>MAHHHHHHIPVTHIKCLRINGQIKCVKPISPNTTPAAEHIEHVRKNPRRKAAMDRA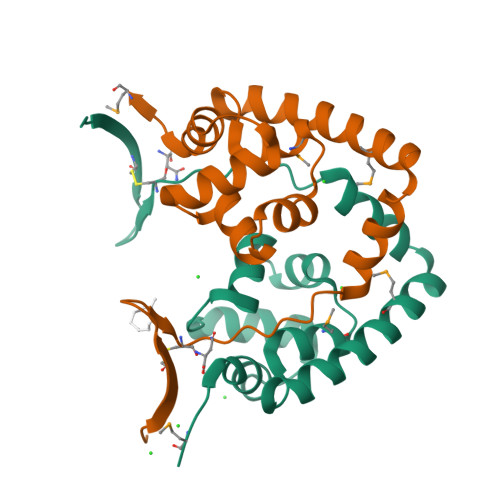AARIADKIALKAGGETFVSLRMKKGFTQSELATAAGLPQPYLSRIENSKQSLQDKTVQKLANALGVSPLEVRAAFERRYEYMEQA[4x]> GASRASRSHSRREEHSGRNGLHHPSPDHFWPRFPDALRPFVPWDQLENEDSSVHISPRQKRDANSSIYKGKKCRMESCFDFTLCKKNGFKVYVYPQQKGEKIAESYQNILAAIEGSRFYTSDPSQACLFVLSLDTLDRDQLSPQYVHNLRSKVQSLHLWNNGRNHLIFNLYSGTWPDYTEDVGFDIGQAMLAKASISTENFRPNFDVSIPLFSKDHPRTGGERGFLKFNTIPPLRKYMLVFKGKRYLTGIGSDTRNALYHVHNGEDVVLLTTCKHGKDWQKHKDSRCDRDNTEYEKYDYREMLHNATFCLVPRGRRLGSFRFLEALQAACVPVMLSNGWELPFSEVINWNQAAVIGDERLLLQIPSTIRSIHQDKILALRQQTQFLWEAYFSSVEKIVLTTLEIIQDRIFKHISRNSLIWNKHPGGLFVLPQYSSYLGDFPYYYANLGLKPPSKFTAVIHAVTPLVSQSQPVLKLLVAAAKSQYCAQIIVLWNCDKPLPAKHRWPATAVPVVVIEGESKVMSSRFLPYDNIITDAVLSLDEDTVLSTTEVDFAFTVWQSFPERIVGYPARSHFWDNSKERWGYTSKWTNDYSMVLTGAAIYHKYYHYLYSHYLPASLKNMVDQLANCEDILMNFLVSAVTKLPPIKVTQKKQYKETMMGQTSRASRWADPDHFAQRQSCMNTFASWFGYMPLIHSQMRLDP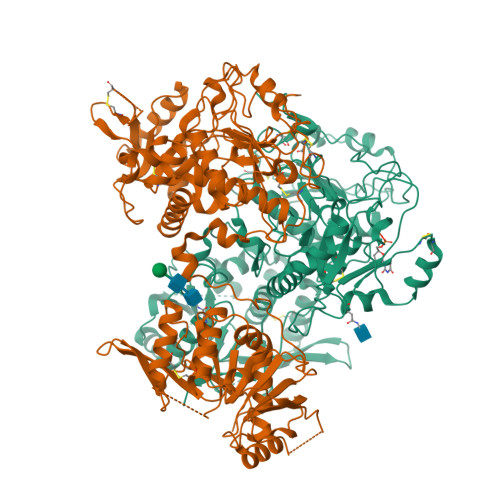VLFKDQVSILRKKYRDIERLNNNNNNGHHHHHHHH;> GASPHSIESSNDWNVEKRSIRDVPVVRLPADSPIPERGDLSCRMHTCFDVYRCGFNPKNKIKVYIYALKKYVDDFGVSVSNTISREYNELLMAISDSDYYTDDINRACLFVPSIDVLNQNTLRIKETAQAMAQLSRWDRGTNHLLFNMLPGGPPDYNTALDVPRDRALLAGGGFSTWTYRQGYDVSIPVYSPLSAEVDLPEKGPGPRQYFLLSSQVGLHPEYREDLEALQVKHGESVLVLDKCTNLSEGVLSVRKRCHKHQVFDYPQVLQEATFCVVLRGARLGQAVLSDVLQAGCVPVVIADSYILPFSEVLDWKRASVVVPEEKMSDVYSILQSIPQRQIEEMQRQARWFWEAYFQSIKAIALATLQIINDRIYPYAAISYEEWNDPPAVKWGSVSNPLFLPLIPPQSQGFTAIVLTYDRVESLFRVITEVSKVPSLSKLLVVWNNQNKNPPEDSLWPKIRVPLKVVRTAENKLSNRFFPYDEIETEAVLAIDDDIIMLTSDELQFGYEVWREFPDRLVGYPGRLHLWDHEMNKWKYESEWTNEVSMVLTGAAFYHKYFNYLYTYKMPGDIKNWVDAHMNCEDIAMNFLVANVTGKAVIKVTPRKKFKCPECTAIDGLSLDQTHMVERSECINKFASVFGTMPLKVVEHRADPVLYKDDFPEKLKSFPNIGSLNNNNNNGHHHHHHHH>GAPSNIAGMIVFLDPGHNGANDASIGRQVPTGRGGTKNCQESGTATDDGYPEHSFTWDTTLRVRAALTALGVRTAMSRGNDNALGPCVDERAAMANSLRPHAIVSIHADGGPPTGRGFHVLYSSPPLNAAQSGPSVQFAKVMRDQLAASGIPPATYIGQGGLNPRSDIAGLNLAQFPSVLVECGNMKNPVDSALMKSPEGRQKYADAIVRGIAGFLGSQSQAAAAVSPVR[2x]

PG remodeling is performed by numerous autolysins acting on specific substrates and at different stages during bacterial growth. While glycosidases, such as muraminidases and glucosaminidases act to hydrolyze the glycosidic bonds between the carbohydrate units, peptidases, such as N-acetylmuramyl-l-alanine amidases, l,d-endopeptidases, d,l-endopeptidases, l,d-carboxypeptidases, and dd-carboxypeptidases, hydrolyze the amide bonds of the peptide stem at specific positions. Ami1Mab and Ami1Msm displayed an overall globular structure comprising a central β-sheet (β1, 4, 5, 6, 7, 8) surrounded by strands β2 and β3 forming an antiparallel β-sheet, six α-helices, and one 310 helix (η1). The catalytic zinc is coordinated by the highly-conserved triad which constitutes the amidase_3 motif signature, namely H25, E60, and H115 in Ami1Mab and H51, E86, and H141 in Ami1Msm.

In addition, to have a complete structural view and to compare the Ami1 structures from M. tuberculosis, M. smegmatis, and M. abscessus, we have also solved the crystal structure of Ami1Msm at a high resolution. Ami1Mab shares 68% and 65% primary sequence identity with Ami1Msm and Ami1Mtb, respectively, while Ami1Msm and Ami1Mtb possess 79% identity. MSMEG_6281 (Ami1Msm), containing an amidase_3 domain, is dispensable for bacterial growth but ami1 deletion mutants present an atypical lateral branching and a defect in cell separation and septal PG turnover. This mutant is also more susceptible to antibiotics due to increased cell wall permeability; a phenotype subsequently confirmed in an independent study which also reported the attenuation of the virulence the ami1 mutant in a mouse model of infection. While cell division was impaired in the ami1Msm knockout strain, this phenotype could be rescued by complementation with the orthologue gene, Rv3717, from M. tuberculosis (ami1Mtb), suggesting a similar mode of action in both species. Furthermore, ami1Msm has also been shown to be important for biofilm formation. In M. smegmatis, deletion of ami1 increases type 3-3 crosslinks as compared to the WT strain.5-(2-fluoro-4-hydroxyphenyl)-1-methyl-1H-pyrrole-2-carbonitrile | C12 H9 F N2 O | 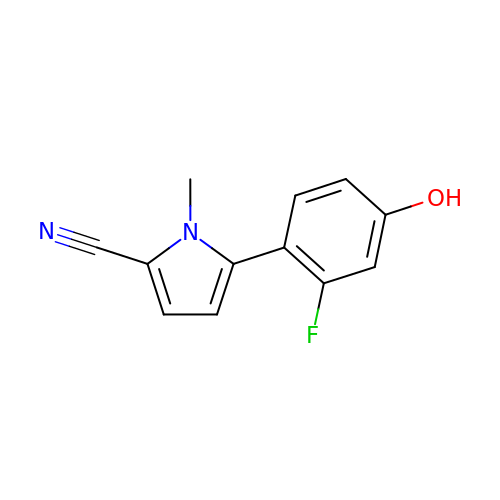WVKAVGHFAICIIO-UHFFFAOYSA-N4-CHLORO-L-PHENYLALANINE | C9 H10 Cl N O2 | 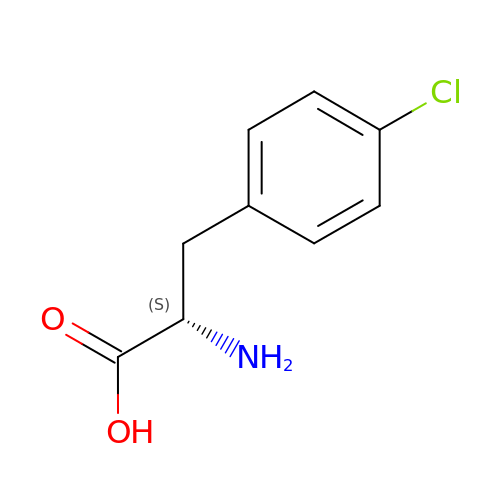NIGWMJHCCYYCSF-QMMMGPOBSA-N> MNIFRLTGDLSHLAAIIILLLKIWKSRSCAGISGKSQLLFALVFTTRYLDLFTSFISLYNTSMKLIYIACSYATVYLIYMKFKAT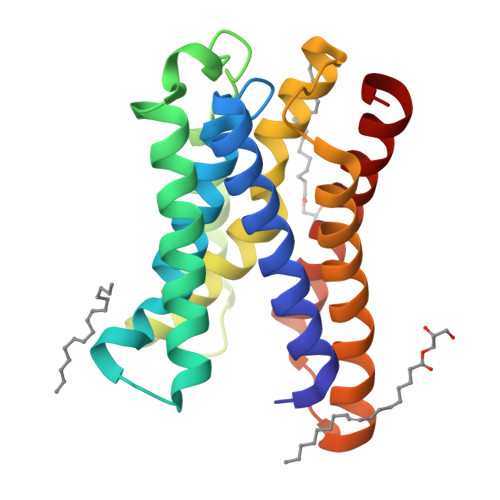YDGNHDTFRVEFLIVPVGGLSFLVNHDFSPLEILWTFSIYLESVAILPQLFMISKTGEAETITTHYLFFLGLYRALYLVNWIWRYYFEGFFDLIAVVAGVVQTVLYCDFFYLYVTKVL> SLTFDHSLEAQWTKWKAMHNRLYGMNEEGWRRAVWEKNMKMIELHNQEYREGKHSFTMAMNAFGDMTSEEFRQVMNGFQNRKPRKGKVFQEPLFYEAPRSVDWREKGYVTPVKNQGQCGSCWAFSATGALEGQMFRKTGRLISLSEQNLVDCSGPQGNEGCNGGLMDYAFQYVQDNG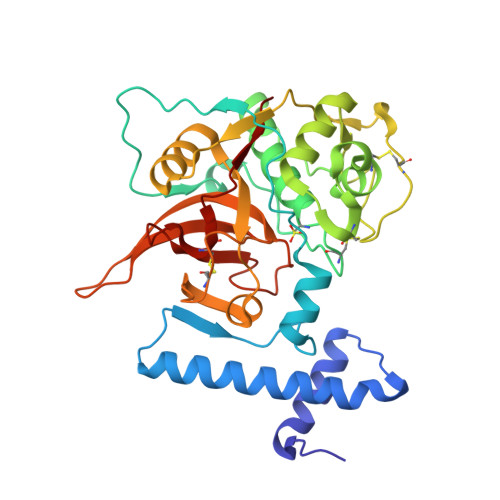GLDSEESYPYEATEESCKYNPKYSVANDAGFVDIPKQEKALMKAVATVGPISVAIDAGHESFLFYKEGIYFEPDCSSEDMDHGVLVVGYGFESTESDNNKYWLVKNSWGEEWGMGGYVKMAKDRRNHCGIASAASYPTV>[5x]MTPQNITDLCAEYHNTQIHTLNDKIFSYTESLAGKREMAIITFKNGATF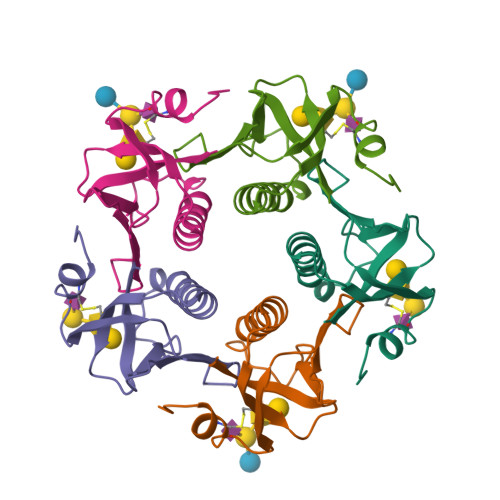QVEVPGSQHIDSQKKAIERMKDTLRIAYLTEAKVEKLCVWNNKTPHAIAAISMAN(1R,2R,3S,4S,5S,6S)-CYCLOHEXANE-1,2,3,4,5,6-HEXOL 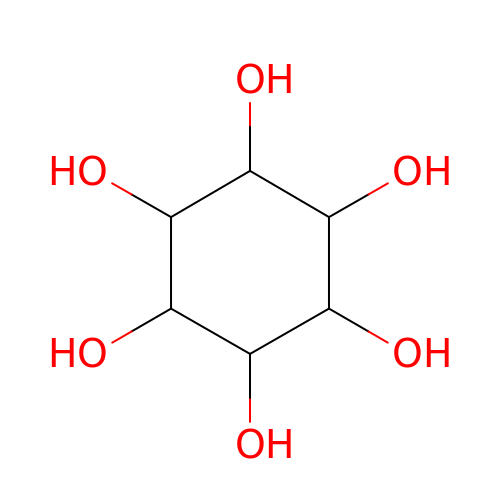| C6 H12 O6 | CDAISMWEOUEBRE-LKPKBOIGSA-N> TTHTSDFLKLNPSSGLWPASG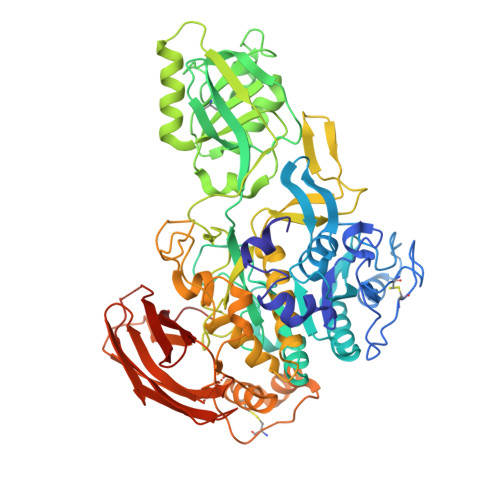LGQDVIVAVLDSGIWPESASFQDDGMPEIPKRWKGICKPGTQFNASMCNRKLIGANYFNKGILANDPTVNITMNSARDTDGHGTHCASITAGNFAKGVSHFGYAPGTARGVAPRARLAVYKFSFNEGTFTSDLIAAMDQAVADGVDMISISYGYRFIPLYEDAISIASFGAMMKGVLVSASAGNRGPGIGSLNNGSPWILCVASGHTDRTFAGTLTLGNGLKIRGWSLFPARAFVRDSPVIYNKTLSDCSSEELLSQVENPENTIVICDDNGDFSDQMRIITRARLKAAIFISEDPGVFRSATFPNPGVVVNKKEGKQVINYVKNSVTPTATITFQETYLDTKPAPVVAASSARGPSRSYLGISKPDILAPGVLILAAYPPNVFATSIGTNILLSTDYILESGTSMAAPHAAGIAAMLKAAHPEWSPSAIRSAMMTTADPLDNTRKPIKDSDNNKAATPLDMGAGHVDPNRALDPGLVYDATPQDYVNLLCSLNFTEEQFKTIARSSASHNCSNPSADLNYPSFIALYSIEGNFTLLEQKFKRTVTNVGKGAATYKAKLKAPKNSTISVSPQILVFKNKNEKQSYTLTIRYIGDEGQSRNVGSITWVEQNGNHSVRSPIVTSPIIEVW>[2x]GLTPEQKQKKAALSASEGEEVPQDKAPSHVPFLLIGGGTAAFAAARSIRARDPGARVLIVSEDPELPYMRPPLSKELWFSDDPNVTKTLRFKQWNGKERSIYFQPPSFYVSAQDLPHIENGGVAVLTGKKVVQLDVRDNMVKLNDGSQITYEKCLIATGGTPRSLSAIDRAGAEVKSRTTLFRKIGDFRSLEKISREVKSITIIGGGFLGSELACALGRKARALGTEVIQLFPEKENMGKILPEYLSNWTMEKVRREGVKVMPNAIVQSVGVSSGKLLIKLKDGRKVETDHIVAAVGLEPNVELAKTGGLEIDSDFGGFRVNAELQARSNIWVAGDAACFYDIKLGRRRVEHHDHAVVSGRLAGENMTGAAKPYWHQSMFWSDLGPDVGYEAIGLVDSSLPTVGVFAKATAQDNPKS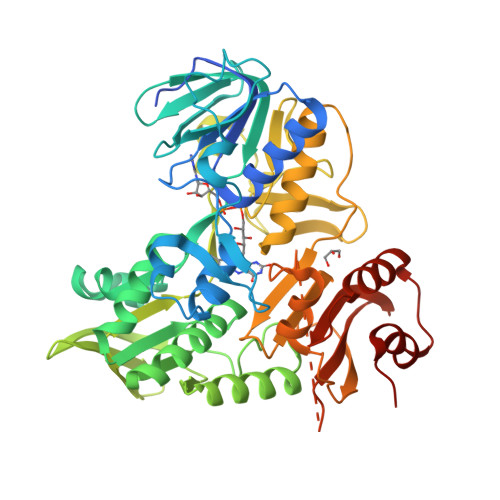ATEQSGTGIRSESETESEASEITIPPSTPAVPQAPVQGEDYGKGVIFYLRDKVVVGIVLWNIFNRMPIARKIIKDGEQHEDLNEVAKLFNIHEDLVPR> SEFMEPLKVEKFATANRGNGLRAVTPLRPGELLFRSDPLAYTVCKGSRGVVCDRCLLGKEKLMRCSQCRVAKYCSAKCQKKAWPDHKRECKCLKSCKPRYPPDSVRLLGRVVFKLMDGAPSESEKLYSFYDLESNINKLTEDRKEGLRQLVMTFQHFMREEIQDASQLPPAFDLFEAFAKVICNSFTICNAEMQEVGVGLYPSISLLNHSCDPNCSIVFNGPHLLLRAVRDIEVGEELTICYLDMLMTSEERRKQLRDQYCFECDCFRCQTQDKDADMLTGDEQVWKEVQESLKKIEELKAHWKWEQVLAMCQAIISSNSERLPDINIYQLKVLDCAMDACINLGLLEEALFYGTRTMEPYRIFFPGSHPVRGVQVMKVGKLQLHQGMFPQAMKNLRLAFDIMRVTHGREHSLIEDL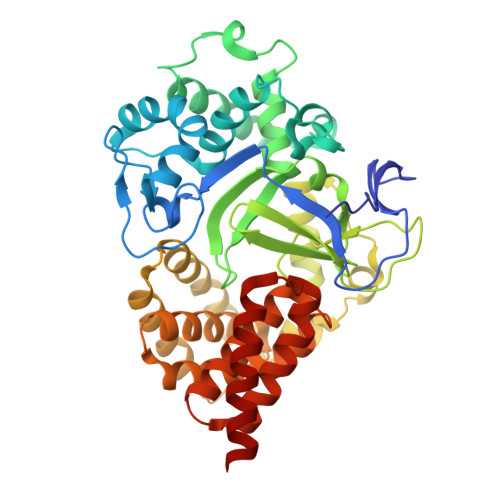ILLLEECDANIRAS>MGSTRLRNASVWLCGLLCLLQVVPSINADVSGCKPGFSSAEYIFSVNRRELERGRKLGKVNFSDCTTRKHGLYDVGDSRFRVLPDGTVLVKRHVKLHKDTKFTISTWDARGIKHSTNIAVASKRHRSGEEAHSRSSKLPVLTFPETHTGLKRKKRDWVIPPIKVSENERGPFPKRLVQIKSNKDRFNKVYYSITGQGADNPPQGVFRIEWETGWMLVTRPLDREEYDKYVLSSHAVSENGSPVEEPMEITINVIDQNDNRPKFTQDVFRGSVREGVQPGTQVMAVSATDEDDNIDSLNGVLSYSILKQDPEEPIPNLFTINRETGVISLIGTGLDREKFPEYTLTVQATDLEGAGLSVEGKAIIQITDANDNAPIFDPKTYTALVPENEIGFEVQRLSVTDLDMPGTPAWQAVYKIRVNEGGFFNITTDPESNQGILTTAKGLDFELRKQYVLQITVENAEPFSVPLPTSTATVTVTVEDVNEAPFFVPAVSRVDVSEDLSRGEKIISLVAQDPDKQQIQKLSYFIGNDPARWLTVNKDNGIVTGNGNLDRESEYVKNNTYTVIMLVTDDGVSVGTGTGTLILHVLDVNDNGPVPSPRVFTMCDQNPEPQVLTISDADIPPNTYP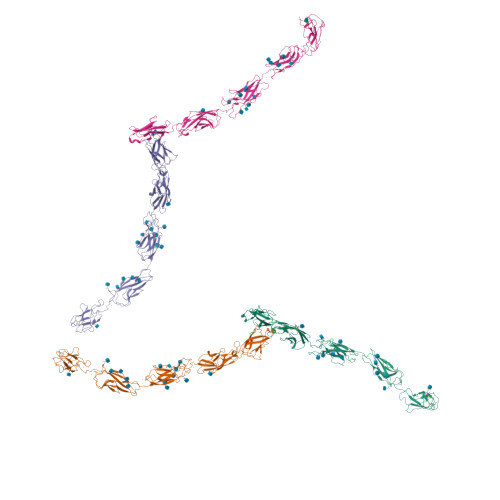YKVSLSHGSDLTWKAELDSKGTSMLLSPTQQLKKGDYSIYVLLSDAQNNPQLTVVNATVCSCEGKAIKCQEKLVGGFDLPIILVILGSVLALLILFLLLLLFLKRKKVVKEPLLLPEDDTRDNIFYYGEEGGGEEDQDYDLSQLHRGLDSRPDIMRNDVVPTLMPAPHYRPRPSNPDEIGNFIDENLDAADNDPTAPPYDSLLVFDYEGSGSEAASLSSLNSSNSNDEHDYNYLSDWGSRFRKLADMYGGDDDEE[4x]>[2x]AAFTQAPMLEQNKQLPPVDQRLPEKPLVIKPIASNGVYGGTLRTVMRGNADGNGILRTIGPQGLTHWTQDIQTVEPYVAESYTVSPDAMEYTFKLRKGMKWSDGTPFTADDIVFAMNDVVLNKEMFPQTPSAYLVGGKAPKVSKVDDYTVKFEFPAANLSFPETLATPLGQHPTLYQKKYCSQFHPAYNKNVQAEFTKANVKDWPSLMRAKCSDIELPSRWSSTERPSIDPWLIKEPYGGAVTRVVMERNPFYWQVDPTGKQLPYVDRIQYAVVSDLQAIILAATNGQYDIEARLLGSDVTSRPLMLKNQQKGGYKVFGQTSANANAAGLWLNQTTKNEKLRKYMTQHDFRQALSLAMDRDEINKVAWLGQAAPWQSGPFKESKWYN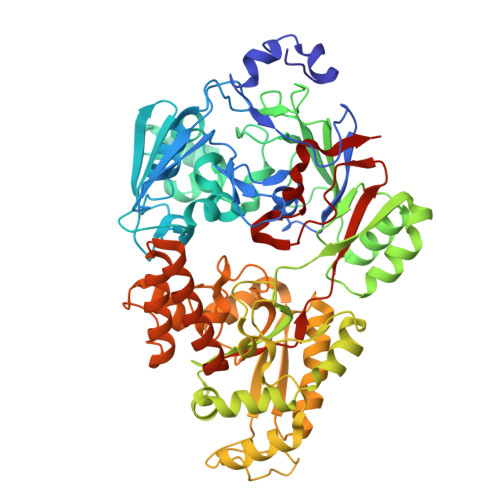EKLATQYLKLDLAQANQILDRLGLTKRDSDGYRTYPDGGRVSLDAIVMIDRQAMVQTLELIRRQWQKAGVELVIKGSERSLFYNRATANDYDISIDVFPGGLDATLNPRAYVAVHPLESRMSLEWAKWYLSGGKQGIEPNESMKKRMALYDQFVAAKTQSQALSLFKQILQISADEFEVIGTVRPAVISSLHSLKLQNVNEKMPFGWPYATPSLSLPQQWYFSKLEHHHHHH Protein arginine methyltransferases (PRMTs) methylate arginine residues in histone and non-histone proteins in a mono, and symmetric or asymmetric dimethyl manner. PRMT7 is a monomethyl arginine methyltransferase that has a role in muscle physiology and stem cell biology. PRMT7, a member of the PRMT family, has been functionally implicated in a wide range of cellular processes including DNA damage signaling, imprinting, and regulation of pluripotency. PRMT enzymes display methylation preference for RGG/RG motifs enriched at protein–protein interfaces, whereas PRMT7 has been reported to target RXR motifs in arginine and lysine-rich regions.

Human PRMT7 shares 93% sequence identity with Mus musculus PRMT7 (MmPRMT7), and the key residues involved in SAM and substrate-binding sites are conserved between the two species. To provide further insight into the mechanism of action of SGC8158, we solved the crystal structure of full-length MmPRMT7 in complex with SGC8158 refined to 2.4 Å resolution (referred to here as MmPRMT7_SGC8158). The structure showed that SGC8158, interacted only with the catalytically active N-terminal methyltransferase domain of PRMT7 in MmPRMT7_SGC8158. Clear electron density was observed for the ribosyl and biphenylmethylamine moieties of SGC8158. The biphenylmethylamine moiety of SGC8158 extends toward the conserved THW loop region (residues Arg311 to Met315) and displaces the Trp314 side chain, to occupy a hydrophobic pocket composed of Trp282, Phe146, Tyr48, Met296, Arg44, and Arg311 side chains, and forms an edge-to-face π-stacking interaction with Trp282. The PRMT-conserved THW loop is part of the active-site pocket and involved in substrate binding, but interestingly SGC8158 did not affect the peptide substrate binding. Comparison of the THW loop region in MmPRMT7 with all other PRMTs showed that this loop has a variable length and conformation, suggesting that it likely has a role in the selectivity of SGC8158 for PRMT7. SGC8158 is a structural derivative of SAM, acts as a SAM-competitive inhibitor of PRMT7, and occupies the adenosine pocket in the SAM-binding site of PRMT7. With increasing concentrations of SAM in the presence of a constant peptide concentration, we observed higher IC50 values, which indicated a SAM-competitive pattern of inhibition. Additional optimization of the methylene linker length between the terminal amine moiety of SGC0911 and the adenosine core structure resulted in SGC8158, a potent PRMT7 inhibitor (IC50 < 2.5 nM), which showed good selectivity over a panel of 35 methyltransferases including PRMTs and kinases.

> MKVFCGRANPTTGSLEWLEEDEHYDYHQEIARSSYADMLHDKDRNIKYYQGIRAAVSRVKDRGQKALVLDIGTGTGLLSMMAVTAGADFCYAIEVFKPMAEAAVKIVERNGFSDKIKVINKHSTEVTVGPDGDLPCRANILITELFDTELIGEGALPSYEHAHKHLVQEDCEAVPHRATVYAQLVESRRMWSWNKLFPVRVRTSLGEQVIVPPSELERCPGAPSVCDIQLNQVSPADFTVLSDVLPMFSVDFSKQVSSSAACHSRQFVPLASGQAQVVLSWWDIEMDPEGKIKCTMAPFWAQTDPQELQWRDHWMQCVYFLPQEEPVVQGSPRCLVAHHDDYCVWYSLQRTSPDENDSAYQVRPVCDCQAHLLWNRPRFGEINDQDRTDHYAQALRTVLLPGSVCLCVSDGSLLSMLAHHLGAEQVFTVESSVASYRLMKRIFKVNHLEDKISVINKRPELLTAADLEGKKVSLLLGEPFFTTSLLPWHNLYFWYVRTSVDQHLAPGAVVMPQAASLHAVIVEFRDLWRIRSPCGDCEGFDVHIMDDMIKHSLDFRESREAEPHPLWEYPCRSLSKPQEILTFDFQQPIPQQPMQSKGTMELTRPGKSHGAVLWMEYQLTPDSTISTGLINPAEDKGDCCWNPHCKQAVYFLSTTLDLRVPLNGPRSVSYVVEFHPLTGDITMEFRLADTLS DEBROMOHYMENIALDISINE | C11 H11 N5 O2 | 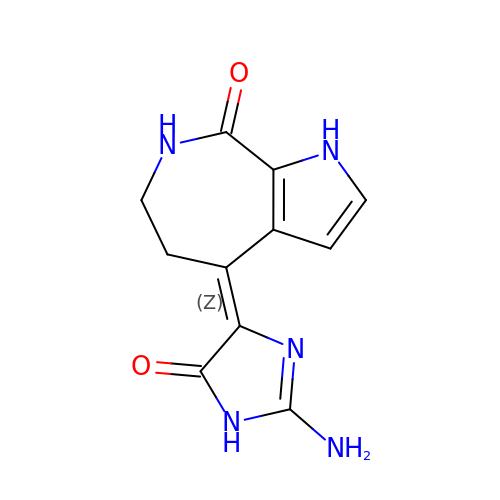JYRJOQGKGMHTOO-VURMDHGXSA-N>ACYCRAPACIAGERRYGTCIYQGRLWAFCC[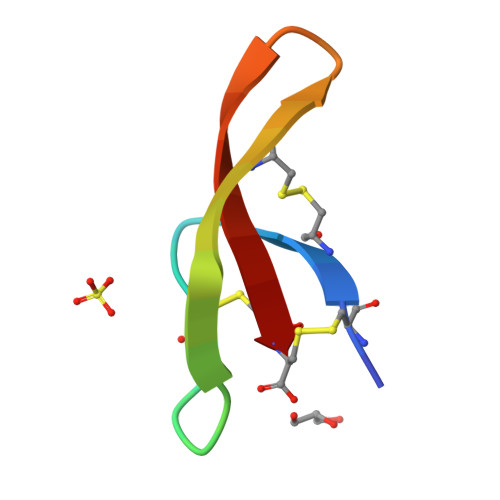2x]> SMKDYDELLKYYELHETIGTGGFAKVKLACHI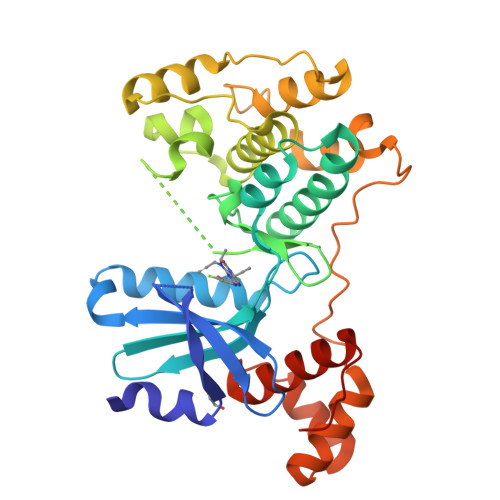LTGEMVAIKIMDKNTLGSDLPRIKTEIEALKNLRHQHICQLYHVLETANKIFMVLEYCPGGELFDYIISQDRLSEEETRVVFRQIVSAVAYVHSQGYAHRDLKPENLLFDEYHKLKLIDFGLCAKPKGNKDYHLQTCCGSLAYAAPELIQGKSYLGSEADVWSMGILLYVLMCGFLPFDDDNVMALYKKIMRGKYDVPKWLSPSSILLLQQMLQVDPKKRISMKNLLNHPWIMQDYNYPVEWQSKNPFIHLDDDCVTELSVHHRNNRQTMEDLISLWQYDHLTATYLLLLAKKARGKPVRLRLSSFS(5S)-5-[(1R)-1-(4-fluoranyl-1H-indol-3-yl)ethyl]-2-(methylamino)-1,3-oxazol-4-one 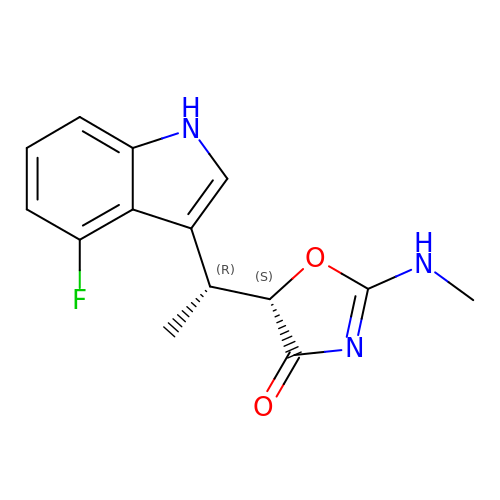| C14 H14 F N3 O2 | RPLLAXTXYOESKS-KRTXAFLBSA-N> MSIVMQLQDVAESTRLGPLSGEVRAGEILHLVGPNGAGKSTLLARMAGMTSGKGSIQFAGQPLEAWSATKLALHRAYLSQQQTPPFATPVWHYLTLHQHDKTRTELLNDVAGALALDDKLGRSTNQLSGGEWQRVRLAAVVLQITPQANPAGQLLLLDQPMCSLDVAQQSALDKILSALSQQGLAIVMSSHDLNHTLRHAHRAWLLKGGKMLASGRREEVLTPPNLAQAYGMNFRRLDIEGHRMLI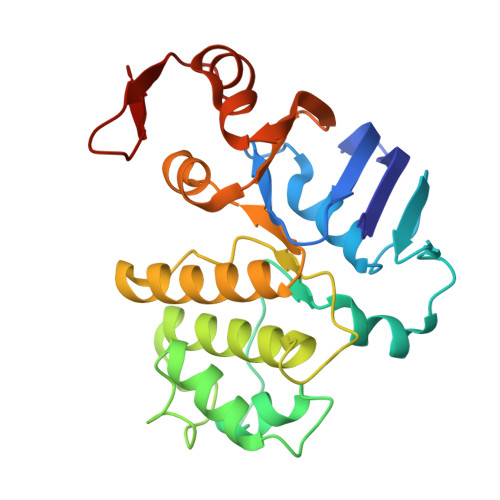STI3-[(4-imidazol-1-yl-6-piperazin-1-yl-1,3,5-triazin-2-yl)amino]-4-methyl-~{N}-[3-(trifluoromethyl)phenyl]benzamide | C25 H24 F3 N9 O | 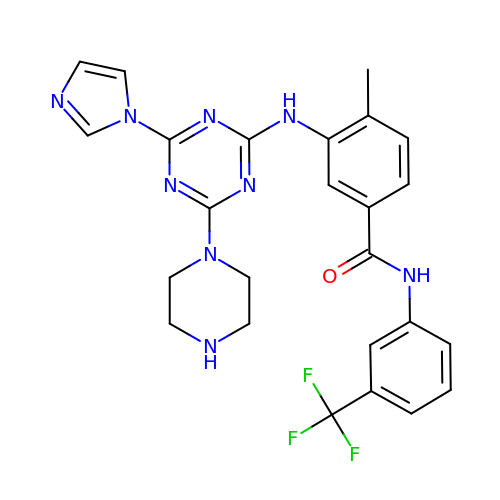NMVJFOBGLWAPPI-UHFFFAOYSA-N> MVEGAVKTEPVDLFHPGFLNSSNYRIPALFKTKEGTLIASIDARRHGGADAPNNDIDTAVRRSEDGGKTWDEGQIIMDYPDKSSVIDTTLIEDDETGRIFLLVTHFPSKYGFWNAGLGSGFKNIDGKEYLCLYDSSGKEFTVRENVVYDKDSNKTEYTTNALGDLFRNGTKIDNINSSTAPLKAKGTSYINLVYSDDDGKTWSEPQNINFQVKKDWMKFLGIAPGRGIQIKNGEHKGRIVVPVYYTNEKGKQSSAVIYSDDSGKNWTIGESPNDNRKLENGKIINSKTLSDDAPQLTECQVVEMPNGQLKLFMRNLSGYLNIATSFDGGATWDETVEKDTNVLEPYCQLSVINYSQKVDGKDAVIFSNPNARSRSNGTVRIGLINQVGTYENGEPKYEFDWKYNKLVKPGYYAYSCLTELSNGNIGLLYEGTPSEEMSYIEMNLKYLES

The genomes of most C. perfringens strains contain three separate genes encoding highly conserved GH33 CAZymes targeting sialic acid glycosidic linkages: the nonsecreted 43 kDa NanH, and the two secreted 77 kDa NanI and 129 kDa NanJ. Here, we present the structural and biochemical characterization of the GH33 catalytic domains of the three sialidases of C. perfringens and probe their substrate specificity. The catalytically active domains, which we refer to as NanHGH33, NanJGH33, and NanIGH33, displayed differential activity on various naturally occurring forms of sialic acid. We report the X-ray crystal structures of these domains in complex with relevant sialic acid variants revealing the molecular basis of how each catalytic domain accommodates different sialic acids.

NanI possess an additional N-terminal family 40 carbohydrate binding module (CBM). However, Neu5Gc (and its alternately acetylated species) is a naturally occurring variant of sialic acid that is present in BSM and was released to some extent by all of the enzymes, though low abundance made it difficult to confidently assign the structures of the acetylated variants. We were able to generate a complex of NanIGH33 with Neu5Gc, which highlighted a “Gc pocket” that can accommodate the additional O11 hydroxyl group of Neu5Gc. This pocket also appears to be present in NanJGH33 and NanHGH33, which is consistent with their ability to release this monosaccharide. Based on the relative abundances of the released Neu5Gc variants, and comparison across the three enzymes, it appears that NanIGH33 is the least able at releasing Neu5Gc, whereas NanJGH33 may be marginally better than NanHGH33. NanIGH33 was most stringent being entirely unable to accommodate 7-O-Ac modification and was comparatively poor at hydrolyzing Neu5Gc variants.> GSAMDSSRRQYQEKYKQVEQYMSFHKLPADFR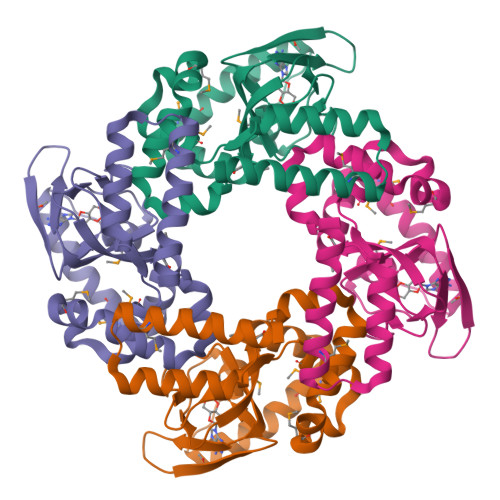QKIHDYYEHRYQGKMFDEDSILGELNGPLREEIVNFNCRKLVASMPLFANADPNFVTAMLTKLKFEVFQPGDYIIREGTIGKKMYFIQHGVVSVLTKGNKEMKLSDGSYFGEICLLTRGRRTASVRADTYCRLYSLSVDNFNEVLEEYPMMRRAFETVAIDRLDRIGKKNSILLH> QYSPNTQQGRTSIVHLFEWRWVDIALECERYLAPKGFGGVQVSPPNENVAIYNPFRPWWERYQPVSYKLCTRSGNEDEFRN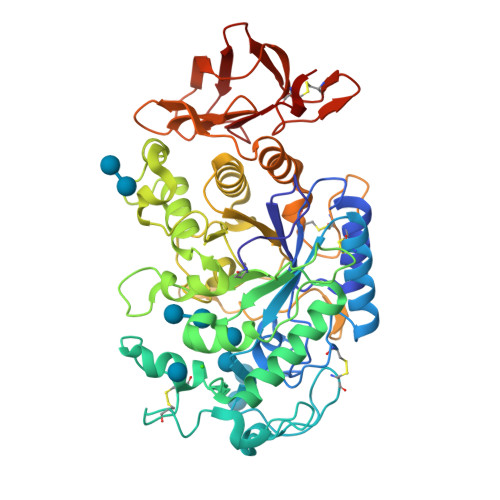MVTRCNNVGVRIYVDAVINHMCGNAVSAGTSSTCGSYFNPGSRDFPAVPYSGWDFNDGKCKTGSGDIENYNDATQVRDCRLTGLLDLALEKDYVRSKIAEYMNHLIDIGVAGFRLDASKHMWPGDIKAILDKLHNLNSNWFPAGSKPFIYQEVIDLGGEPIKSSDYFGNGRVTEFKYGAKLGTVIRKWNGEKMSYLKNWGEGWGFMPSDRALVFVDNHDNQRGHGAGGASILTFWDARLYKMAVGFMLAHPYGFTRVMSSYRWPRQFQNGNDVNDWVGPPNNNGVIKEVTINPDTTCGNDWVCEHRWRQIRNMVIFRNVVDGQPFTNWYDNGSNQVAFGRGNRGFIVFNNDDWSFSLTLQTGLPAGTYCDVISGDKINGNCTGIKIYVSDDGKAHFSISNSAEDPFIAIHAESKL>[3x]FVEMVDNLRGKSGQGYYVEMTVGSPPQTLNILVDTGSSNFAVGAAPHPFLHRYYQRQLSSTYRDLRKGVYVPYTQGKWEGELGTDLVSIPHGPNVTVRANIAAITESDKFFINGSNWEGILGLAYAEIARPDDSLEPFFDSLVKQTHVPNLFSLQLCGAGFPLNQSEVLASVGGSMIIGGIDHSLYTGSLWYTPIRREWYYEVIIVRVEINGQDLKMDCK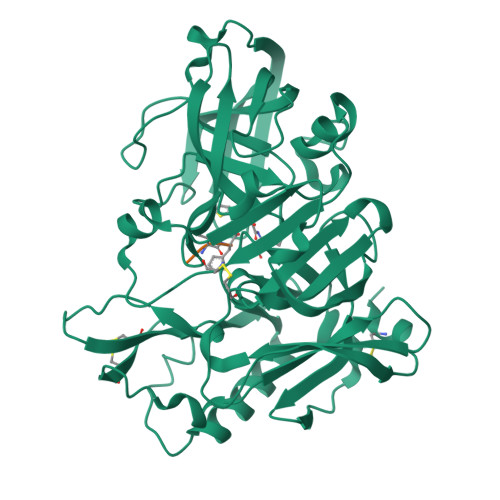EYNYDKSIVDSGTTNLRLPKKVFEAAVKSIKAASSTEKFPDGFWLGEQLVCWQAGTTPWNIFPVISLYLMGEVTNQSFRITILPQQYLRPVEDVATSQDDCYKFAISQSSTGTVMGAVIMEGFYVVFDRARKRIGFAVSACHVHDEFRTAAVEGPFVTLDMEDCGYNI> MSSSAPKYTTFQGSQNFRLRIVLATLSGKPIKIEKIRSGDLNPGLKDYEVSFLRLIESVTNGSVIEISYTGTTVIYRPGIIVGGASTHICPSSKPVGYFVEPMLYLAPFSKKKFSILFKGITASHNDAGIEAIKWGLMPVMEKFGVRECALHTLKRGSPPLGGGEVHLVVDSLIAQPITMHEIDRPIISSITGVAYSTRVSPSLVNRMIDGAKKVLKNLQCEVNITADVWRGENSGKSPGWGITLVAQSKQKGWSYFAEDIGDAGSIPEELGEKVACQLLEEISKSAAVGRNQLPLAIVYMVIGKEDIGRLRINKEQIDERFIILLRDIKKIFNTEVFLKPVDEADNEDMIATIKGIGFTNTSKKIA;> WNIGKLIYMDNISPEECIRRWRGEDDDSKDESDIEEDVDDDFFRKKDGTVTKEGNKDHAVDLEKFVPYFDTFEK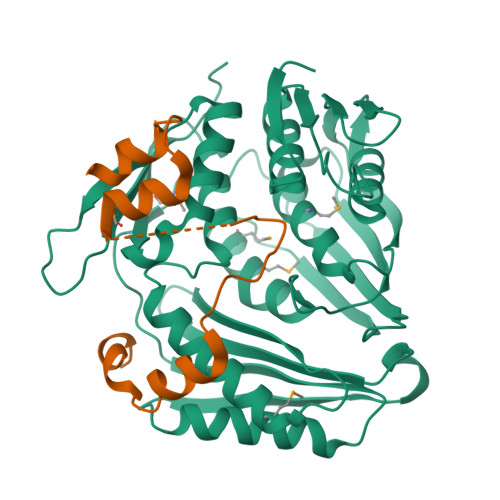LAKKWKSVDAIKERFL>MPDLNSIAALRQVQTRSISPENFDGTAGGGGRATEGTGADCARDLGPGWKISPSVDIKAGETFELASIEGAGKITHIWITTHTDNWRTLILRAFWDGADEPAVEVPYGDFFCNGWGVFAQVNSQAIAANPHGGFNSYWPMPFRDGARLTIENTSVVDVRVYYQVTYEIGGDHSNDAYFHAQW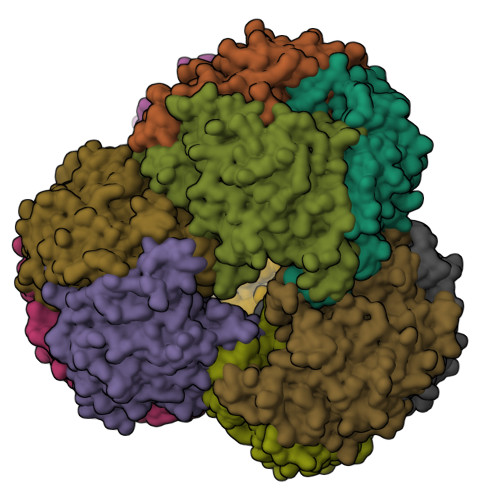RRSNPLEELTPHVILEGIEGEGHYVGTYIAWGVNSNGWWGEGEIKFYLDDDTDHPTICGTGTEDYFGGAWNFDIPGKGYTEFSTPYLGMPQVIRPDGLYVSQQRFGMYRWHLQDPIHFATGIPKVDIQALGWRSGWRYLPLRDDIASTAMFYLDRPTARRPKSPSADDMEVHLGTAPVPDLGATPPRVLEHHHHHH[12x]>[2x]ACRQEPQPQGPPPAAGAVASYDYLVIGGGSGGLASARRAAELGARAAVVESHKLGGTCVNVGCVPKKVMWNTAVHSEFMHDHADYGFPSCEGKFNWRVIKEKRDAYVSRLNAIYQNNLTKSHIEIIRGHAAFTSDPKPTIEVSGKKYTAPHILIATGGMPSTPHESQIPGASLGITSDGFFQLEELPGRSVIVGAGYIAVEMAGILSALGSKT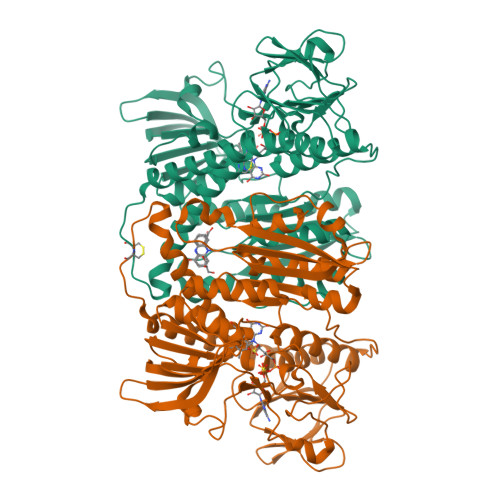SLMIRHDKVLRSFDSMISTNCTEELENAGVEVLKFSQVKEVKKTLSGLEVSMVTAVPGRLPVMTMIPDVDCLLWAIGRVPNTKDLSLNKLGIQTDDKGHIIVDEFQNTNVKGIYAVGDVCGKALLTPVAIAAGRKLAHRLFEYKEDSKLDYNNIPTVVFSHPPIGTVGLTEDEAIHKYGIENVKTYSTSFTPMYHAVTKRKTKCVMKMVCANKEEKVVGIHMQGLGCDEMLQGFAVAVKMGATKADFDNTVAIHPTSSEELVTLR>MGSSHHHHHHSSGENLYFQGHMALVLDGRALAKQIEENLLVRVEALKAKTGRTPILATILVGDDGASATYVRMKGNACRRVGMDSLKIELPQETTTEQLLAEIEKLNANPDVHGILLQHPVPAQIDERACFDAISLAKDVDGVTCLGFGRMAMGEAAYGSATPAGIMTILKENNIEIAGKHAVVVGRSAILGKPMAMMLLQANATVTICHSRTQNLPELVKQADIIVGAVGKAELIQKDWIKQGAVVVDAGFHPRDGGGVGDIQLQGIEEIASAYTPV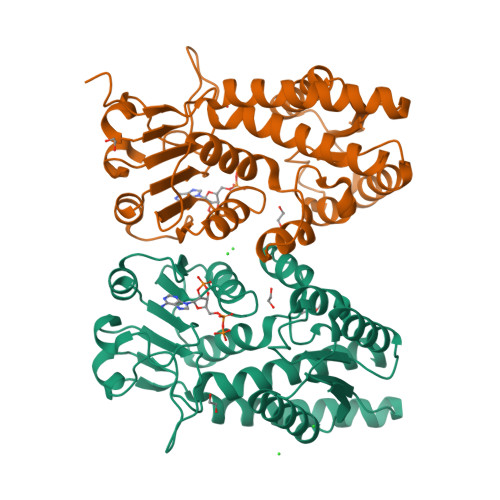PGGVGPMTITTLIRQTVEAAEKALG[2x]>PKDNNKTLKPAIAEYIVKKAKQRIALQRWQDELNRRKNHKGMIFVENTVDLEGPPSDFYYINEYKPAPGISLVNEATFGCSCTDCFFQKCCPAEAGVLLAYNKNQQIKIPPGTPIYECNSRCQCGPDCPNRIVQKGTQYSLCIFRTSNGRGWGVKTLVKIKRMSFVMEYVGEVITSEEAERRGQFYDNKGITYLFDLDYESDEFTVDAARYGNVSHFVNHSCDPNLQVFNVFI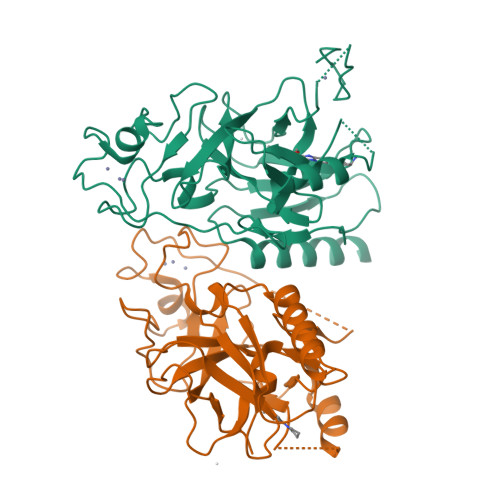DNLDTRLPRIALFSTRTINAGEELTFDYQMKGSGDISSDSIDHSPAKKRVRTVCKCGAVTCRGYLN[2x]> GSAKDPMQIVSINVGKPKTIEVNGERLVTGIDKTPVAHPVAVGKQNLAGDGQADLVHHGGEDKAICAYPSEHFVYWEER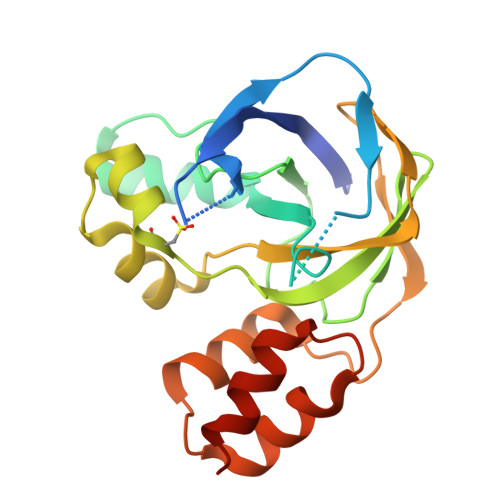YGRPFTAGAFGENWTLLGLTEDDVCLGDIYVAGTALVQVSQPRQPCSKLAFKHQLPDLPKAICQTGKSGFYFRVLQEGVIEPGAPLVLVERGVGALSIAYINHIYYHERDNAAAMKQIASHPALSASWRETFQKRLADRPRP>GSHMLFDFENDQVPSNIHFLNARASIETYTGINGEPSKGLKLAMQSKQHSYTGLAIVPEQPWDWSEFTSASLYFDIVSVGDHSTQFYLDVTDQNGAVFTRSIDIPVGKMQSYYAKLSGHDLEVPDSGDVNDLNLASGLRSNPPTWTSDDRQFVWMWGVKNLDLSGIAKISLSVQSAMHDKTVIIDNIRIQPNPPQDENFLVGLVDEFGQNAKVDYKGKIHSLEELHAARDVELAELDGKPMPSRSKFGGWLAGPKLKATGYFRTEKINGKWMLVDPEGYPYFATGLDIIRLSNSSTMTGYDYDQATVAQRSADDVTPEDSKGLMAVSEKSFATRHLASPTRAAMFNWLPDYDHPLANHYNYRRSAHSGPLKRGEAYSFYSANLERKYGETYPGSYLDKWREVTVDRMLNWGFTSLGNWTDPAYYDNNRIPFFANGWVIGDFKTVSSGADFWGAMPDVFDPEFKVRAMETARVVSEEIKNSPWCVGVFIDNEKSFGRPDSDKAQYGIPIHTLGRPSEGVPTRQAFSKLLKAKYKTIAALNNAWGLKLSSWAEFDLGVDVKALPVTDTLRADYSMLLSAYADQYFKVVHGAVEHYMPNHLYLGARFPDWGMPMEVVKAAAKYADVVSYNSYKEGLPKQKWAFLAELDKPSIIGEFHIGAMDHGSYHPGLIHAASQADRGEMYKDYMQSVIDNPYFVGAHWFQ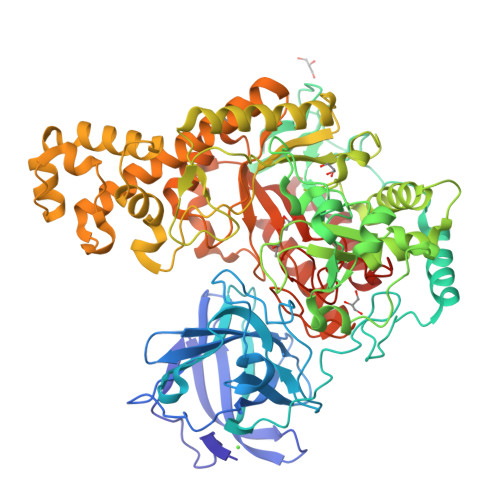YMDSPLTGRAYDGENYNVGFVDVTDTPYQEMVDAAKEVNAKIYTERLGSK[4x]The ProQ/FinO family of RNA binding proteins mediate sRNA-directed gene regulation throughout gram-negative bacteria. The RocC/RocR system regulates competence, a specialized physiological state involving the coordinated expression of multiple genes which allows the bacteria to uptake environmental DNA and integrate it into its chromosome (i.e., natural transformation). RocC binds and stabilizes RocR, which in turn binds and represses a series of mRNA targets that encode components of the DNA uptake system.

We carried out further truncations to define a minimal RNA-binding region of RocC that would be amenable to structural studies. Limited proteolysis suggested RocC24-126 is a stable folded core, however, this construct was defective in interacting with RocRSL3 and could not replace RocC in an in vivo assay to measure DNA uptake efficiency. In contrast, RocC14-126 displayed a similar binding affinity to RocC1-126 and is perfectly functional in vivo, indicating that residues 14–23 contain critical residues for its interaction with RocR. Deletion of the N-terminal 13 residues, which are disordered in our structures, did not impact RNA-binding affinity or transformation repression. However further deletion to residue 24 resulted in a ~threefold reduction in binding affinity, similar to what we had observed by EMSA, and a total loss of transformation repression.

>[2x]GPLGSARSDALLWLAANFPEAFDNSLRIRPLKIGIMSDILQHAEKAEQVGVSKSKLREAVVLFTRRLDYLACLKAREVRIDLHGNPVAEVTEEEAENASMKIKKRVEK> MRYRPFGSTGVAVSA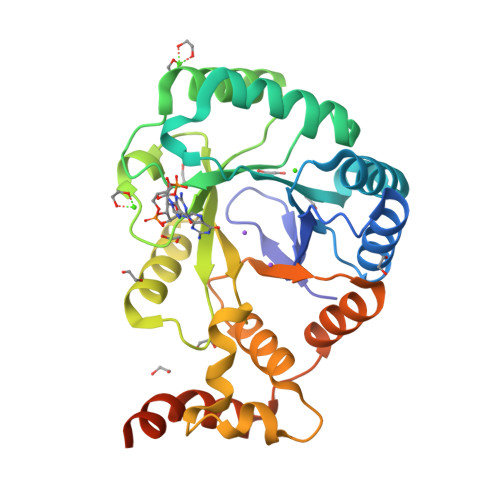LTLRLADNPRLRANDWRALVFTALENGVNSFQIDGDAPELLKGAGEAFASVERHLLFLTWRLRGDAKQLGPHTLDALKRSAFEGLSLDYLDLLLINDPQSASLPMAFESGLQDLQKGRALRGLGVASRGDIDPGLLANDLVTAVSSPYNLSSGWAERHRIRQASQNNFAVIGEDFWPQALRELADVGGYEFLTNTPGWSAEDICLGYALTEPSLATVRVTADNRQEIERLAAVVERDLPTGVCAQIEMARFSAQEREKAARRPKLAAALEHHHHHH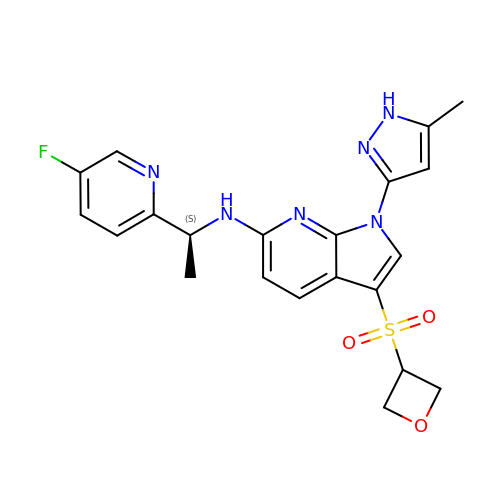N-[(1S)-1-(5-fluoropyridin-2-yl)ethyl]-1-(5-methyl-1H-pyrazol-3-yl)-3-[(oxetan-3-yl)sulfonyl]-1H-pyrrolo[2,3-b]pyridin-6-amine | C21 H21 F N6 O3 S | NNWRFTLSEJKLQI-ZDUSSCGKSA-N During the late phase of HIV-1 infection, viral Gag polyproteins are targeted to the plasma membrane (PM) for assembly. Gag localization at the PM is a prerequisite for the incorporation of the envelope protein (Env) into budding particles. Gag assembly and Env incorporation are mediated by the N-terminal myristoylated matrix (MA) domain of Gag. Pioneering X-ray crystallography studies of HIV-1 unmyristoylated MA [myr(–)MA] revealed that the protein adopts a trimer arrangement.

When mapped on the putative hexamer of trimer model of MA, these residues were found to point toward the hexamer centers. It was also shown that substitution of residue Gln63 with Arg suppressed Env incorporation defects of the L13E, E17K, L31E, V35E, or E99V MA mutations and of a gp41CT mutation that has the same phenotype. To explain the role of MA trimerization in Env incorporation, it was suggested that the Q63R mutation in MA may stabilize the trimer structure such that MA lattices that form large hexamer holes are favored over those that feature small hexamer holes. However, it is not clear how this substitution can stabilize the trimer form. To be able to assess the structural changes in the MA trimer, we determined the high-resolution structure of myr(–)MA Q63R protein by X-ray crystallography. Interestingly, the two crystal forms of myr(–)MA Q63R yielded structures that are essentially identical with slightly different parameters. Each asymmetric unit of the crystal structure contains two trimers. The structure of the myr(–)MA Q63R trimer in both crystal forms is virtually identical to that of the WT myr(–)MA protein with slight orientation differences of monomers in the trimeric assembly. The structures in the two crystal forms revealed only minor conformational changes in the loops connecting helices I and II and helices V and VI. Intriguingly, the guanidinium group of Arg63 is 2.5 Å (averaged across 12 examples in the asymmetric unit of the two crystal forms) from the hydroxyl group of Ser67 of an adjacent MA molecule, which forms new hydrogen bonding in the trimer interface. Our findings complemented the biological data by showing that the H-bond formed between the side chains of Arg63 and Ser67 is key for the stability of the MA trimer and hence to its function in rescuing Env incorporation.

>[6x]GARASVLSGGELDKWEKIRLRPGGKKQYKLKHIVWASRELERFAVNPGLLETSEGCRQILGRLQPSLQTGSEELRSLYNTIAVLYCVHQRIDVKDTKEALDKIEEEQNKSKKKAQQAAADTGNNSQVSQNYHHHHHH>[2x]MLNQFPGQYSNNIFCFPPIESETKSGKKASWIICVQVVQHNTIIPITDEMFSTDVKDAVAEIFTKFFVEEGAVRISKMTRVTEGKNLGKKNATTVVHQAFKDALSKYNRHARQKRGAHTNRGMIPPMLVKYFNIIPKTFFEEETDPIVQRKRNGVRAVACQQGDGCILLYSRTEKEFLGLDNIKKELKQLYLFIDVRVY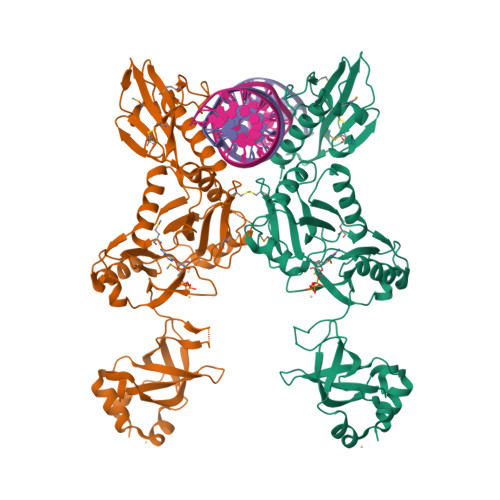LDGELYLHRKPLQWIAGQANAKTDSSELHFYVFDCFWSDQLQMPSNKRQQLLTNIFKQKEDLTFIHQVENFSVKNVDEALRLKAQFIKEGYEGAIVRNANGPYEPGYNNYHSAHLAKLKPLLDAEFILVDYTQGKKGKDLGAILWVCELPNKKRFVVTPKHLTYADRYALFQKLTPALFKKHLYGKELTVEYAELSPKTGIPLQARAVGFREPINVLEII>[2x]MTTLTRADWEQRAQNLKIEGRAFIQGEYTAAASGETFDCISPVDGRLLAKVASCDAADAQRAVESARSAFDSGAWSRLAPAKRKATMIRFAGLLEQNAEELALLETLDMGKPISDSLGVDIPGGARALSWSGE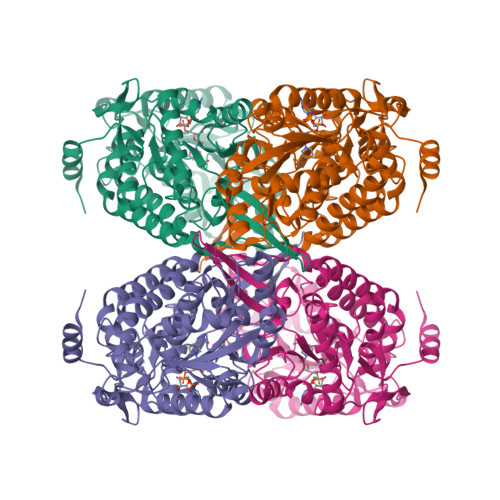AIDKLYDEVAATPHDQLGLVTREPVGVVAAIVPWNFPLMMACWKLGPALSTGNSVVLKPSEKSPLTAIRIAQLAIEAGIPAGVLNVLPGYGHTVGKALALHMDVDTVVFTGSTKIAKQLMIYAGESNMKRVWLEAGGKSPNIVFADAPDLQAAADSAASAIAFNQGEVCTAGSRLLVERSIKDRFLPMVIEALGTWKPGNPLDPATNVGALVDTQQMNTVLSYIAAGHTDGARLVAGGKQILQETGGTYVEPTIFDGVNNAMRIAQEEIFGPVLSVLTFDTAEEAIQIANDTPYGLAAAVWTANLSKAHLTARALRAGSVWVNQYDGGDMTAPFGGFKQSGNGRDKSLHAFDKYTELKSTWIKL>KGGEKTDIKQVPWTVAVRTYPGEESLTCGGAILSQWFVLTAAHCVFDQKPETIVIQYESTNLWEDPGKSDPYVSHVYLSFYRQETMENDIAILELSRPLKLDGLKSKPAKLPDIEFRPKTGSDVLVSGYGDGQTMDPKDHDLKSAQLTVVDLDECRTKYGPIFLSLQVFCAQKVGVSLE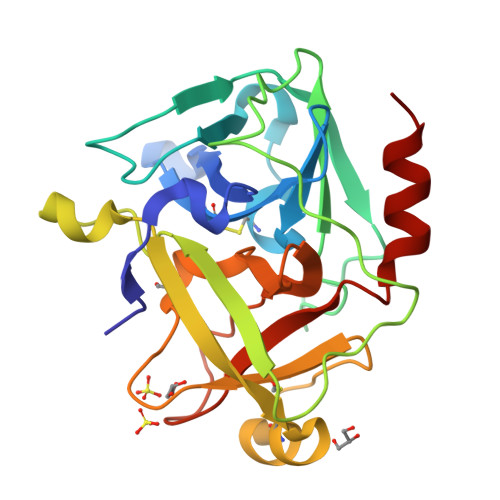SGDAGDPTVQQDTLVGVAAYFPKRPEGAPEVFTKVGSYVSWIQDIIKKK[2x]>NAILADRSTSALYVRVGEQLHPVLNLTSARLISGSPDNPTMVKTSEIDKFPRGNLLGIPGAPERMVQNAATDAEWTVCDAVGGANPGVTVIAGPLGADGERAAPLPPDHAVLVHSDAEPNPGDWLLWDGKRSPIDLADRAVTDALGLGGQALAPRPIAAGLFNAVPAAP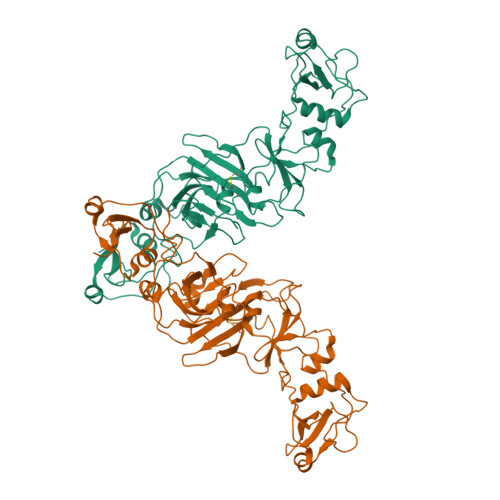ALTAPVIPDAGAAPQFELSLPVPVGAVVVAYDADNTARYYAVLSDGLQPISPVLAAILRNTDSHGFAQPPRLGPDEVARTPMSRGLDTSAYPDNPVTLVEASAHPVTCAHWTKPSDAAESSLSVLSGAVLPLAEGLHTVDLVGAGAGGAANRVALTPGTGYFVQTVGAEPGSPTAGSMFWVSDTGVRYGIDTAEDDKVVAALGLSTSPLPVPWSVLSQFAAGPALSRGDALVAHDAVSTNPNSARMEASR[2x]>[2x]MEEHTQGSHVEAGIVEHPNAEDFGHARTLPTDTNWFKHAVFYEVLVRAFYDSNADGIGDLRGLTE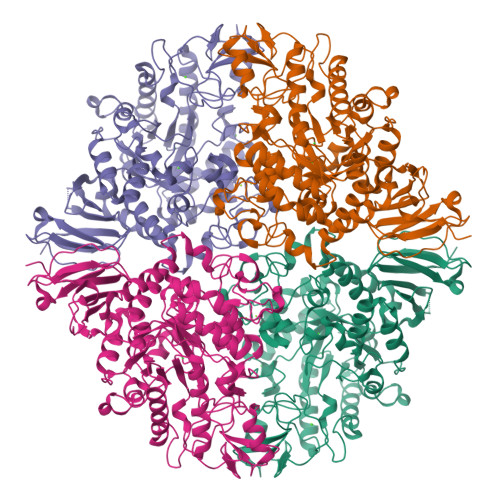KLDYIKWLGVDCLWLPPFYDSPLRDGGYDIRDFYKVLPEFGTVDDFVTLLDAAHRRGIRIITDLVMNHTSDQHEWFQESRHNPDGPYGDFYVWSDTSDRYPDARIIFVDTEESNWTFDPVRRQFYWHRFFSHQPDLNYDNPAVQEAMLDVLRFWLDLGIDGFRLDAVPYLFEREGTNCENLPETHAFLKRCRKAIDDEYPGRVLLAEANQWPADVVAYFGDPDTGGDECHMAFHFPLMPRIFMAVRRESRFPISEILAQTPPIPDTAQWGIFLRNHDELTLEMVTDEERDYMYAEYAKDPRMKANVGIRRRLAPLLENDRNQIELFTALLLSLPGSPVLYYGDEIGMGDIIWLGDRDSVRTPMQWTPDRNAGFSKATPGRLYLPPNQDAVYGYHSVNVEAQLDSSSSLLNWTRNMLAVRSRHDAFAVGTFRELGGSNPSVLAYIREVTRQQGDGGAKTDAVLCVNNLSRFPQPIELNLQQWAGYIPVEMTGYVEFPSIGQLPYLLTLPGHGFYWFQLREPDPEPGAQQ>MGNTVMKNCNYKRKRRERDWDCNTKKDVCIPDRRYQLCMKELTNLVNNTDTNFHRDITFRKLYLKRKLIYDAAVEGDLLLKLNNYRYNKDFCKDIRWSLGDFGDIIMGTDMEGIGYSKVVENNLRSIFGTDEKAQQRRKQWWNESKAQIWTAMMYSVKKRLKGNFIWICKLNVAVNIEPQIYRWIREWGRDYVSELPTEVQKLKEKCDGKINYTDKKVCKVPPCQNACKSYDQWITRKKNQWDVLSNKFISVKNAEKVQTAGIVTPYDILKQELDEFNEVAFENEINKRDGAYIELCVCSVEEAKKNTQ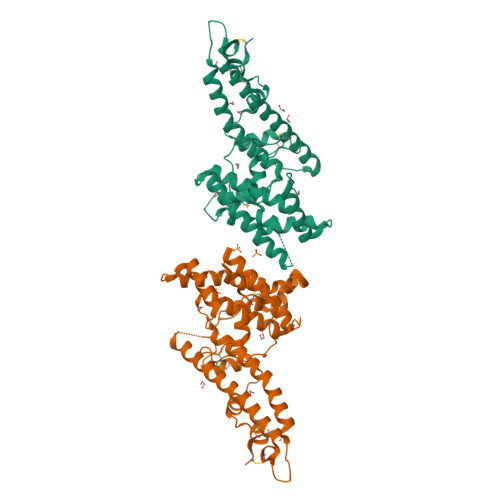EVVTNVDN[2x]>[2x]MTVQMEYEKDVKVAALDGKKIAVIGYGSQGHAHAQNLRDSGRDVIIGVRPGKSFDKAKEDGFDTYTVAEATKLADVIMILAPDEIQQELYEAEIAPNLEAG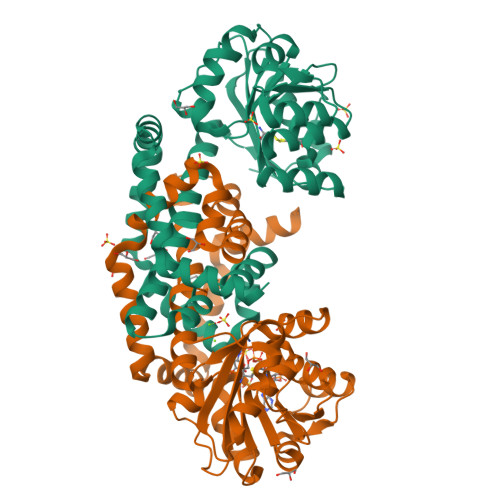NAVGFAHGFNIHFEFIKVPADVDVFMCAPKGPGHLVRRTYEEGFGVPALYAVYQDATGNAKNIAMDWCKGVGAARVGLLETTYKEETEEDLFGEQAVLCGGLTALIEAGFEVLTEAGYAPELAYFEVLHEMKLIVDLIYEGGFKKMRQSISNTAEYGDYVSGPRVITEQVKENMKAVLADIQNGKFANDFVNDYKAGRPKLTAYREQAANLEIEKVGAELRKAMPFVGKNDDDAFKIYN Norrie Disease Protein (NDP) gene encodes Norrin, a secreted cystine-knot like growth factor, distinct from the lipid-modified Wnt. Unlike Wnts which have promiscuous interactions with Fz receptors, Norrin specifically binds to Fz4CRD, but not to the 14 other CRDs of Fz and secreted Frizzled-related protein (sFRP) family members. The Norrin mediated pathway maintains the blood-retina and blood-brain barriers and regulates angiogenesis in the cochlea and uterus as well as neuroprotective effects on retinal neurons. Our crystallographic and solution studies further reveal that dimeric Norrin forms a complex with two copies of monomeric Fz4CRD.

We purified Norrin–Fz4CRD complex and determined the crystal structures of methylated Norrin–Fz4CRD (dimethylated surface-exposed lysine residues) and Norrin–Fz4CRD–SOS (complex bound with heparin mimic sucrose octasulfate, SOS) at 2.3 Å and 3.0 Å resolution, respectively. These two complex structures show different stoichiometries: a 2:1 complex for the methylated Norrin–Fz4CRD and a 2:2:2 stoichiometry for the Norrin–Fz4CRD–SOS complex, the architecture of which resembles a butterfly. To investigate the preference for complex formation in a 2:1 or 2:2 stoichiometry, we performed SEC-MALS and SAXS measurements in the absence of SOS. Both methods show Norrin interacts with Fz4CRD in a 2:2 stoichiometry. Lysine methylation of the Norrin–Fz4CRD complex was used to facilitate crystal lattice formation, and on close inspection of the structure we found Lys102 and Lys104, two residues which contribute to the Norrin–Fz4CRD interface, (see next section) are dimethylated in the uncomplexed subunit of the Norrin dimer, and contribute instead to a lattice contact. This observation suggests that the 2:1 stoichiometry merely reflects the favourable crystallization characteristics of a sub population of asymmetrically methylated Norrin–Fz4CRD complexes. Thus although the methylated Norrin–Fz4CRD structure usefully provides high-resolution information for the ligand–receptor interface, the Norrin–Fz4CRD–SOS structure defines the overall architecture of the native complex. The Norrin–Fz4CRD binding interface is conserved between the complex structures. Each Fz4CRD interacts one-to-one with a separate Norrin chain, burying on average 1680 Å2 of surface area. At the ligand–receptor interface two β-hairpins in Norrin (β1-β2 and β5-β6) contact three loops in Fz4CRD (I, II, and III).

>GPGKTDSSFIMDSDPRRCMRHHYVDSISHPLYKCSSKMVLLARCEGHCSQASRSEPLVSFSTVLKQPFRSSCHCCRPQTSKLKALRLRCSGGMRLTATYRYILSCHCEECNSGTETSQVAPA[2x];> DTGERRCDPIRISMCQNLGYNVTKMPNLVGHELQTDAELQLTTFTPLIQYGCSSQLQFFLCSVYVPMCTEKINIPIGPCGGMCLSVKRRCEPVLKEFGFAWPESLNCSKFPPQNDHNHMCMEGPGDEEVPLPHKTPIQPGEGTLEVLFQ> MSLFGTTSGFGTSGTSMFGSATTDNHNPMKDIEVTSSPDDSIGCLSFSPPTLPGNFLIAGSWANDVRCWEVQDSGQTIPKAQQMHTGPVLDVCWSDDGSKVFTASCDKTAKMWDLSSNQAIQIAQHDAPVKTIHWIKAPNYSCVMTGSWDKTLKFWDTRSSNPMMVLQLPERCYCADVIYPMAVVATAERGLIVYQLENQPSEFRRIESPLKHQHRCVAIFKDKQNKPTGFALGSIEGRVAIHYINPPNPAKDNFTFKCHRSNGTNTSAPQDIYAVNGI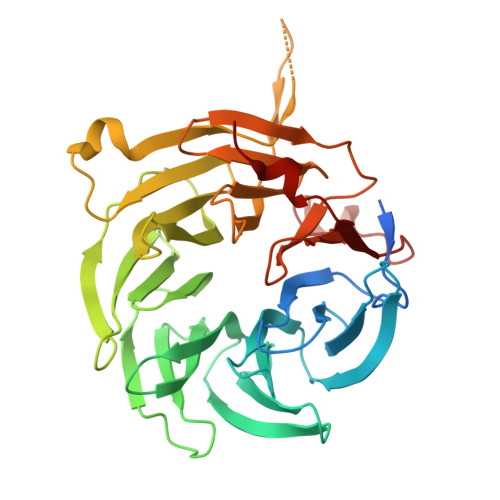AFHPVHGTLATVGSDGRFSFWDKDARTKLKTSEQLDQPISACCFNHNGNIFAYASSYDWSKGHEFYNPQKKNYIFLRNAAEELKPRNKK>[3x]QDSTSDLIPAPPLSKVPLQQNFQDNQFHGKWYQVGRAGNAALREDKDPQ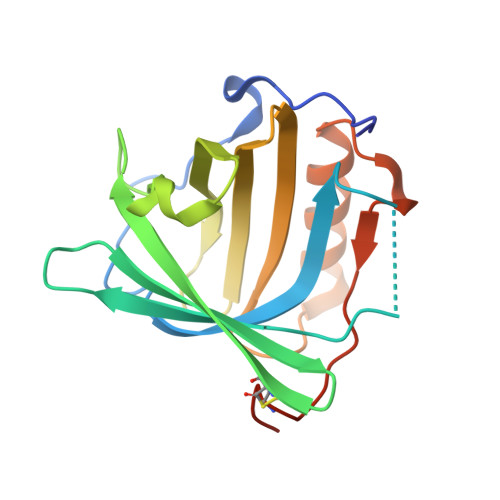KMTAQIYELKEDKSYNVTAVRFRKKKCDYATMTFVPGSQPGEFTLGNIKSYPGLTSYLVRVVSTNYNQHAMVFFKKVSQNREYFSITLLGRTKELASELKENFIRFSKSLGLPENHIVFPVPIDQCIDGSAHHHHHH>[2x]MPIHDHDHPFHGYQLEKEP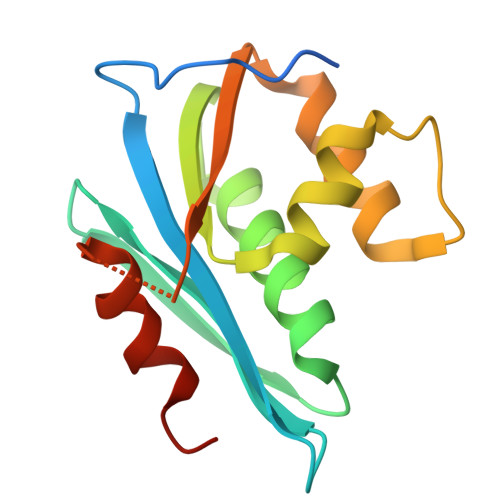IVGAETFYVDGAANRETKLGKAGYVTNKGRQKVVPLTNTTNQKTELQAIYLALQDSGLEVNIVTDSQYALGIIQAQPDKSESELVNQIIEQLIKKEKVYLAWVPAHKGIGGNEQVDKLVSAGIRKIL>GPGSMIHPMAVDRLLPSQEAAELIELTREIADKVLDPIVDRHEKDETYPEGVFE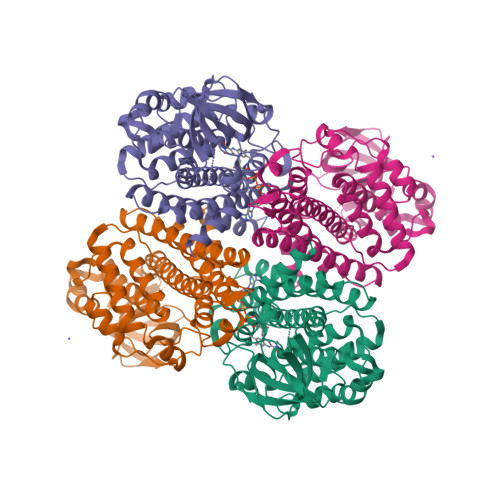QLGAAGLLSLPQPEEWGGGGQPYEVYLQVLEEIAARWASVAVAVSVHSLSSHPLLVFGTEEQKKRWLPGMLSGEQIGAYSLSEPQAGSDAAALRCAATPTDGGYVINGSKSWITHGGKADFYTLFARTGEGSRGVSCFLVPADQPGLSFGKPEEKMGLHAVPTTSAFYDNARIDADRRIGEEGQGLQIAFSALDSGRLGIAAVATGLAQAALDEAVAYANERTAFGRKIIDHQGLGFLLADMAAAVATARATYLDAARRRDQGRPYSQQASIAKLTATDAAMKVTTDAVQVFGGVGYTRDYRVERYMREAKIMQIFEGTNQIQRLVIARGLTR[2x]>MVQKESQATLEERESELSSNPAASAGASLEPPAAPAPGEDNPAGAGGAAVAGAAGGARRFLCGVVEGFYGRPWVMEQRKELFRRLQKWELNTYLYAPKDDYKHRMFWREMYSVEEAEQLMTLISAAREYEIEFIYAISPGLDITFSNPKEVSTLKRKLDQVSQFGCRSFALLFDDIDHNMCAADKEVFSSFAHAQVSITNEIYQYLGEPETFLFCPTEYCGTFCYPNVSQSPYLRTVGEKLLPGIEVLWTGPKVVSKEIPVESIEEVSKIIKRAPVIWDNIHANDYDQKRLFLGPYKGRSTELIPRLKGVLTNPNCEFEANYVAIHTLATWYKSNMNGVRKDVVMTDSEDSTVSIQIKLENEGSDEDIETDVLYSPQMALKLALTEWLQEFGVPHQYSSRQVAHSGAKASVVDGTPLVAAPSLNATTVVTTVYQEPIMSQGAALSGEPTTLTKEEEKKQPDEEPMDMVVEKQEETDHKNDNQILSEIVEAKMAEELKPMDTDKESIAESKSPEMSMQEDCISDIAPMQTDEQTNKEQFVPGPNEKPLYTAEPVTLEDLQLLADLFYLPYEHGPKGAQMLREFQWLRANSSVVSVNCKGKDSAKIAEWRSRAAKFEEMCGLVMGMFTRLSNCANRTILYDMYSYVWDIKSIMSMVKSFVQWLGCRSHSSAQFLIGDQEPWAFRGGLAGEFQRLLPIDGANDLFFQPPPLTPTSKVYTIRPYFPKDEASVYKICREMYDDGVGLPFQSQPDLIGDKLVGGLLSLSLDYCFVLEDEDGICGYALGTVDVTPFIKKCKISWIPFMQEKYTKPNGDKELSEAEKIMLSFHEEQEVLPETFLANFPSLIKMDIHKKVTDPSVAKSMMACLLSSLKANGSRGAFCEVRPDDKRILEFYSKLGCFEIAKMEGFPKDVVILGRSL[2x]

The regulation of O-GlcNAc cycling on thousands of nuclear and cytoplasmic proteins is coordinated by two enzymes. O-GlcNAc transferase (OGT) catalyses the addition of GlcNAc, derived from UDP-GlcNAc, to serine and threonine residues, and O-GlcNAcase (OGA; CAZY database family GH84) cleaves O-GlcNAc. Composed of two ordered domains, the N-terminal glycoside hydrolase domain forms a (β/α)8 barrel, while the C-terminal stalk domain is composed of six α-helices. α17, consisting of Glu676–Pro694, undergoes a dimer ‘swap’, playing a structural role that contributes to dimerization. Structural characterization of the human O-GlcNAcase orthologue (HsOGA-L/HsOGA) showed dimer formation both in solution and in the crystal where it has been shown to be promoted by helix-exchange in contrast to the non-helix-exchanged bacterial dimers.

Surface-entropy reduction (SER) is a concept in which flexible, solvent-exposed residues, primarily lysine and glutamate, are mutated to alanine to reduce the entropic loss during the packing of the protein into a crystalline lattice. Following the co-expression strategy of Roth et al. using pACYC-Duet-1 Gly11–Gln396 and pET-YSBLIC3C Lys535–Tyr715 plasmids, the successful pair of mutations was Glu602Ala/Glu605Ala (HsOGAE602AE605A). Therefore, crystallization conditions were re-screened using the HsOGAE602AE605A variant; crystals were obtained in 17% polyethylene glycol 3350, 0.2 M sodium citrate pH 8.0. The space group was P3121, which is a lower symmetry group compared with P43212 for the HsOGA11–396+535–715 structure. However, the structure was determined to a resolution of 3.3 Å, which was a lower resolution compared with the HsOGA11–396+535–715 and catalytically inactive mutant structures, possibly owing to the thin-rod crystal morphology compared with the large trigonal bi­pyramid wild-type crystals. Unlike HsOGA11–396+535–715, the C-terminus of monomer A can be traced into the active site of the symmetry-related monomer A, with Lys713 binding in the position of O-GlcNAc. Hence, the C-terminus binds to the active site of the symmetry-related monomer A rather than monomer B (as in the wild type). The C-terminus of monomer B could not be built in from Pro707, indicating that it does not bind into an active site because of the crystal packing.> MSLTTYDTQPSTLIRNAAAIMTGGRGTADDPSRVPGPDIRIVGDTIDAIGALAPRPGETIVDATDCVIYPAWVNTHHHLFQSLLKGEPAGLDATLTPWLAATPYRFRALFDERRFRLAARIGLIELARSGCATVADHNYVYYPGMPFDSSAILFEEAEKLGLRFVLLRGGATQTRQLEADLPTALRPETLDAYVADIERLAARYHDASPRAMRRVVMAPTTVLYSISPREMRETAAVARRLGLRMHSHLSETVGYQDSAYSMYGKSPVAFCGEHDWLGSDVWYAHLVKVDADEIALLAQTGTGVAHCPQSNGRLGSGICPVREMADAGVPVSIGVDGAASNEAADMISEV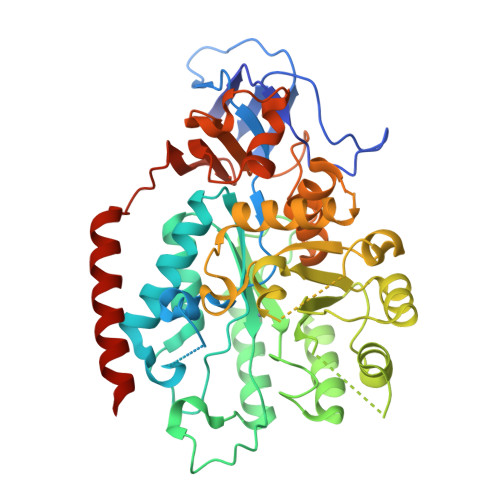HMTWLAQRARLGMLAQPAYRGGSFEGGAGAASIAEVIHWGTAGGARVMGLDEVGKVAVGYAADIAVYRLDDPRYFGLHDPAIGPVASGGRPSVMALFSAGKRVVVDDLIEGVDIKELGGEARRVVRELLREVVVEGHHHHHH(2P)-5-fluoro-2-(1H-pyrazol-5-yl)pyridine 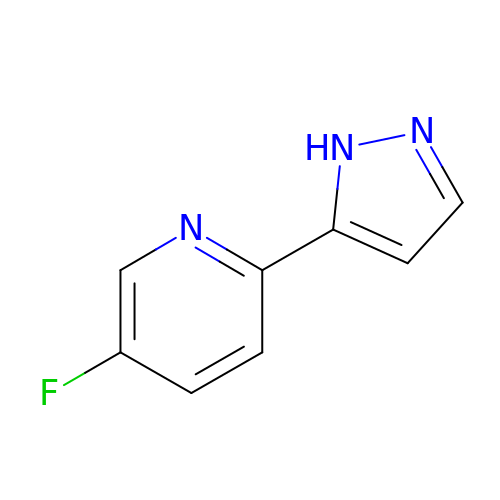| C8 H6 F N3 | ADBMBWBQQBJNNZ-UHFFFAOYSA-N> GGTGGGGCTAGCCCCACC

Nine new crystal structures of CG-rich DNA 18-mers with the sequence 5′-GGTGGGGGC-XZ-GCCCCACC-3′, which are related to the bacterial repetitive extragenic palindromes, are reported. All 18-mers crystallized as isomorphic tetragonal crystals with one strand of a right-handed antiparallel duplex in the asymmetric unit. All reported structures co-crystallized with the Sr2+ cation located between nucleotides 6 and 7 and (by symmetry) 12 and 13.

All four Chom-18-mers with two central nucleotides (residues 9 and 10) able to form Watson–Crick pairs were crystallized. Base pairs A–T and T–A are classified as Watson–Crick pairs, while the C–G pair adopts a specific orientation characterized by a large value of one of the base parameters, shear (2.97 Å), and is not classified.>[2x]SNAMDYQTIPS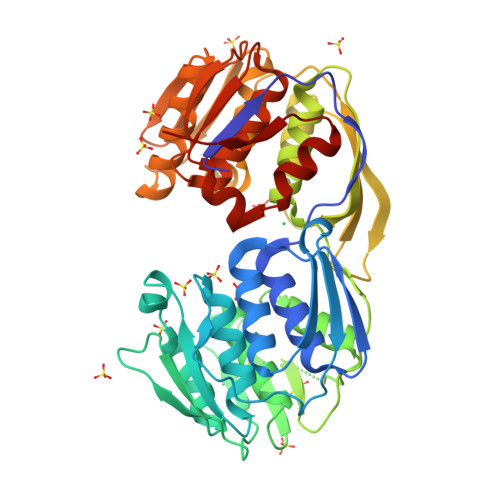QGLSGEICVPGDKSISHRAVLLAAIAEGQTQVDGFLMGADNLAMVSALQQMGASIQVIEDENILVVEGVGMTGLQAPPEALDCGNSGTAIRLLSGLLAGQPFNTVLTGDSSLQRRPMKRIIDPLTLMGAKIDSTGNVPPLKIYGNPRLTGIHYQLPMASAQVKSCLLLAGLYARGKTCITEPAPSRDHTERLLKHFHYTLQKDKQSICVSGGGKLKANDISIPGDISSAAFFIVAATITPGSAIRLCRVGVNPTRLGVINLLKMMGADIEVTHYTEKNEEPTADITVRHARLKGIDIPPDQVPLTIDEFPVLLIAAAVAQGKTVLRDAAELRVKETDRIAAMVDGLQKLGIAAESLPDGVIIQGGTLEGGEVNSYDDHRIAMAFAVAGTLAKGPVRIRNCDNVKTSFPNFVELANEVGMNVKGVRGRGGF> GAMAGTPHIAILPSPGMGHLIPMAEFAKRLVHHHNFSITFVIPTDGPPSSAYQQVLTSLPSSIDHIFLPQVDLTDVVSQSPAHPRIETLISLTVARSLSSLRTTLSSLQSSKNLVSLVVDLFGTDAFDPAIELGISPYIFFPSTAMTLSLFLYMPQLDKSVTCEFRHMTDLVRIPGCVPVRGSDLFDPVQDRTDEAYKWVIHHSNRYPMAEGVIENSFMELEHGALKYLQTVQSGKPPVYAVGPLIKMDYDVDDSGSKIIEWLDDQPVGSVLFVSFGSGGTLSYEQMTELAHG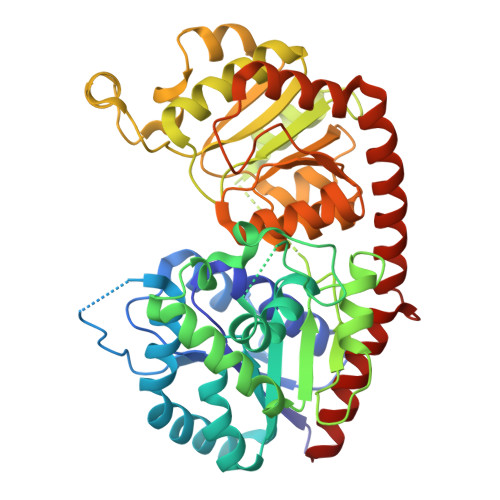LESSQQRFLWVVRSPNQIPNSTYFSVQSQKDPLAYLPEGFLNRTEGRGLVVSNWAPQAQILSHGSTGGFMSHCGWNSILESVVHGVPIIAWPLYAEQKMNSIIVVEDVKVALRPAGVGERVVERSEITAVVKALMEGEEGKKVRNRMKELKEAAARAVSDDGASTIAIADLAQKWRSSMKH>[2x]ADPGSEDCSKNFTSPNGTIESPGFPEKYPHNLDCTFTILAKPKMEIILQFLIFDLEHDPLQVGEGDCKYDWLDIWDGIPHVGPLIGKYCGTKTPSELRSSTGILSLTFHTDMAVAKDGFSARYYLVHQEPLENFQCNVPLGMESGRIANEQISASSTYSDGRWTPQQSRLHGDDNGWTPNLDSNKEYLQVDLRFLTMLTAIATQGAI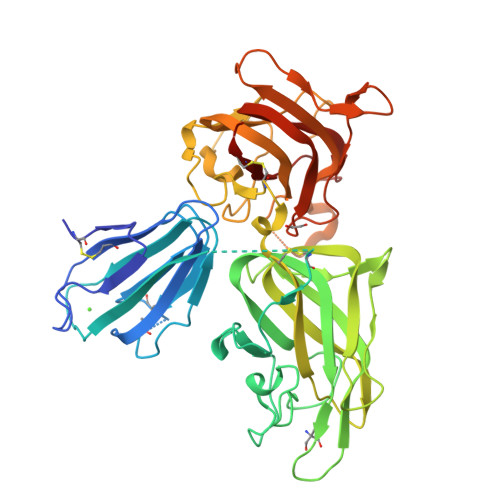SRETQNGYYVKSYKLEVSTNGEDWMVYRHGKNHKVFQANNDATEVVLNKLHAPLLTRFVRIRPQTWHSGIALRLELFGCRVTDAPCSNMLGMLSGLIADSQISASSTQEYLWSPSAARLVSSRSGWFPRIPQAQPGEEWLQVDLGTPKTVKGVIIQGARGGDSITAVEARAFVRKFKVSYSLNGKDWEYIQDPRTQQPKLFEGNMHYDTPDIRRFDPIPAQYVRVYPERWSPAGIGMRLEVLGCDWTHHHHHH>[2x]HEYDVGKLKVEHPWLRAPADGEKNAS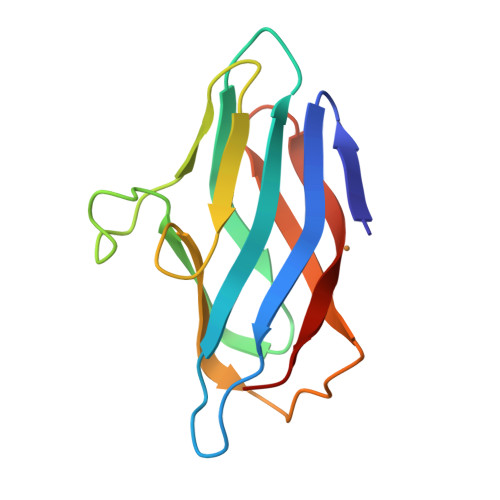FYAFIHNNGDTPDKLVAVKVEKFGSAVIHGDAKNLALEAPVLLPPKQKITLAPGGAYVALLDAKKHLEVGWGLEMTLVFEKAGEVVIDAAIDAPD>MGVFMEKLKTYLELIRVKNCITASIGGIIGYLISSNFEIDILKSLLVFFVVFFVCAYGNVINDIFDIEIDRINK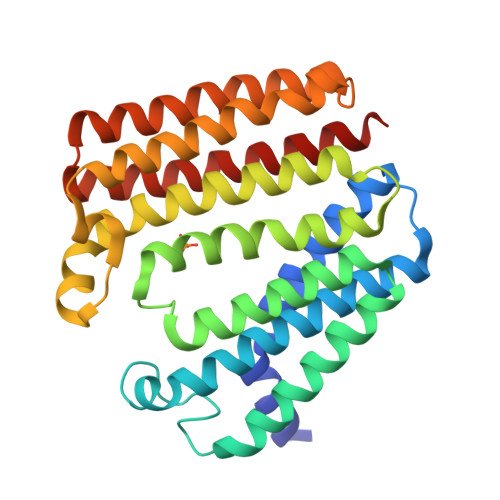PSRPLPSGKIKLNEAKKFSAILLILGLVLSLFINIYALIIAVINALFLYLYAKKYKKYKPIGNFIIGYLTGSVFLFGGVAGKNVMPVVILFLCSLLSIWGREIVKDFEDMEGDKKEGVISLPIKYGKKSLYFATFLVVLAVILSPLPYILKIFGIWYLILIAICDILFIYAMALLLKEPNKETASKVSKFLKIIMNIVLLAFIVGAIKL[2x]> MASSHHHHHHSSGLVPRGSSGSSMAARPPRAKPAPRRRAAQPSDASPAAQVDLRTLGYSQQQQEKIKPKVRSTVAQHHEALVGHGFTHAHIVALSQHPAALGTVAVTYQHIITALPEATHEDIVGVGKQWSGARALEALLTDAGELRGPPLQLDTGQLVKIAKRGGVTAMEAVHASRNALTGAPLNLTPAQVVAIASNNGGKQALETVQRLLPVLCQAHGLTPAQVVAIASHDGGKQALETMQRLLPVLCQAHGLPPDQVVAIASNIGGKQALETVQRLLPVLCQAHGLTPDQVVAIASHGGGKQALETVQRLLPVLCQAHGLTPDQVVAIASHDGGKQALETVQRLLPVLCQAHGLTPDQVVAIAS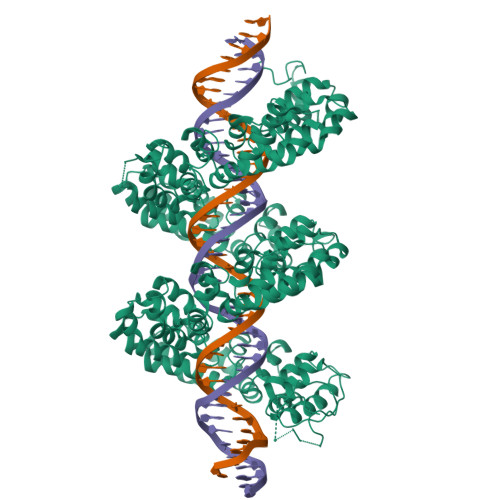NGGGKQALETVQRLLPVLCQAHGLTPDQVVAIASNGGKQALETVQRLLPVLCQAHGLTPDQVVAIASHDGGKQALETVQRLLPVLCQTHGLTPAQVVAIASHDGGKQALETVQQLLPVLCQAHGLTPDQVVAIASNIGGKQALATVQRLLPVLCQAHGLTPDQVVAIASNGGGKQALETVQRLLPVLCQAHGLTPDQVVAIASNGGGKQALETVQRLLPVLCQAHGLTQVQVVAIASNIGGKQALETVQRLLPVLCQAHGLTPAQVVAIASHDGGKQALETVQRLLPVLCQAHGLTPDQVVAIASNGGGKQALETVQRLLPVLCQAHGLTQEQVVAIASNNGGKQALETVQRLLPVLCQAHGLTPDQVVAIASNGGGKQALETVQRLLPVLCQAHGLTPAQVVAIASNIGGKQALETVQRLLPVLCQDHGLTLAQVVAIASNIGGKQALETVQRLLPVLCQAHGLTQDQVVAIASNIGGKQALETVQRLLPVLCQDHGLTPDQVVAIASNIGGKQALETVQRLLPVLCQDHGLTLDQVVAIASNGGKQALETVQRLLPVLCQDHGLTPDQVVAIASNSGGKQALETVQRLLPVLCQDHGLTPNQVVAIASNGGKQALESIVAQLSRPDPALAALTNDHLVALACLGGRPAMDAVKKGLPHAPELIRRVNRRIGERTSHRV>MSDSHHKPVWDRTHHAKMATGIGDPQCFKGMAGKSKFNVGDRVRIKDLPDLFYTRTMTYTRGATGTIVRLVYESPAAEDEAFGNEENVEWFYSIVFAQKDLWPEYSDTFANDTLETEIPERYLEKA[4x];>MSSSIREEVHRHLGTVALMQPALHQQTHAPAPTEITHTLFRAYTRVPHDVGGEADVPIEYHEKEEEIWELNTFATCECLAWRGVWTAEERRRKQNCDVGQTVYLGMPYYGRWLLTAARILVDKQFVTLTELHNKIVEMRERVASGQGLGEYLPPKAK[4x];>[4x]MSADHDHDHDHDHDHKPAPMVEEVSDFEILEMAVRELAIEKGL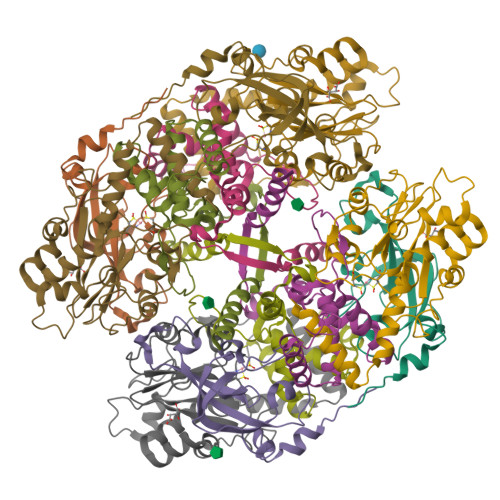FSAEDHRVWKDYVHTLGPLPAARLVAKAWLDPEYKKLCIEDGVEASKAVGVNWVTSPPTQFGTPSDYCNLRVLADSPTLKHVVVCTLCSCYPRPILGQSPEWYRSPNYRRRLVRWPRQVLAEFGLQLPSEVQIRVADSNQKTRYIVMPVRPEGTDGWTEDQLAEIVTRDCLIGVAVPKPGITVNAKRPVLKANRPVHHDH>[2x]GAMGGWAIAVHGGAGVDPTLPLERQEEAKQLLTRCLNLGISALNSNVPAIDVVELVVRELETDPLFNSGRGSAL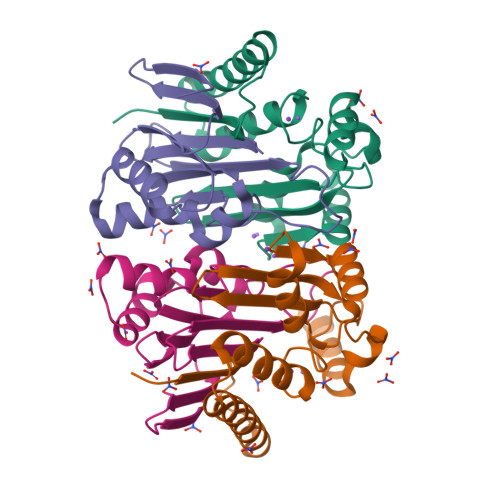TEKGTVEMEASIMDGPKRRCGAVSGLTTVKNPISLARLVMDKSPHSYIAFSGAEDFARQQGVEVVDNEYFVTPDNVGMLKLAKEANTILFDYRIPSSAYETCGSGVESPLQMNGLPISVYAPE;>[2x]TVGCVVVDREGRCAAATSTGGLMNKMTGRIGDSPLIGAGTYACDVCGVSCTGEGEAIIRGTLAREVAAVMEYKGLKLHQAVDFVIKHRLDEGKAGLIAVSNTGEVACGFNCNGMFRACATEDGFMEVAIWD1-(2,5-dichloro-3-{[5-chloro-1-(2H-pyrazolo[3,4-b]pyridin-3-ylmethyl)-1H-benzotriazol-4-yl]oxy}phenyl)methanamine 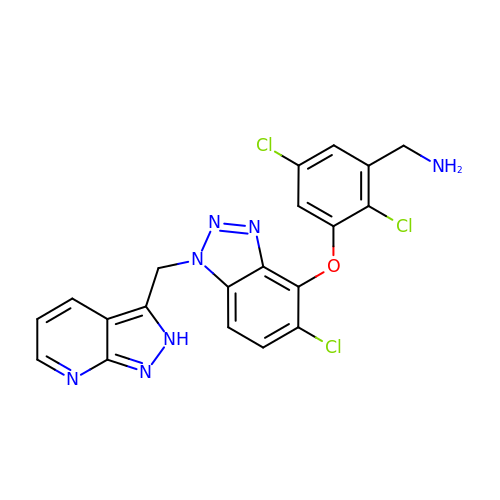| C20 H14 Cl3 N7 O | CUYHWBGVPXGMKQ-UHFFFAOYSA-N(1S,2S)-2-ethyl-1-({[(3aS,4S,6R,7aS)-6-ethyl-1-oxooctahydro-1H-inden-4-yl]carbonyl}amino)cyclopropanecarboxylic 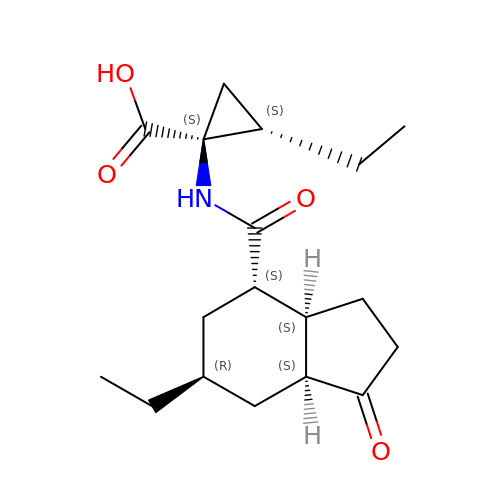acid | C18 H27 N O4 | YYTFHRRGIDEJIS-FNEQEMTHSA-N> IIGGQDAAHGAWPWMVSLQIFTYHNNRRYHVCGGSLLNSQWLLTAAHCFRIKKKVTDWRLIFGAKEVEWGTNKPVKPPLQERYVEKIIIHEKYSASSEANDIALMKITPPVTCGHFIGPGCLPQFRAGPPRVPQTCWVAGWGFLQENARRTSP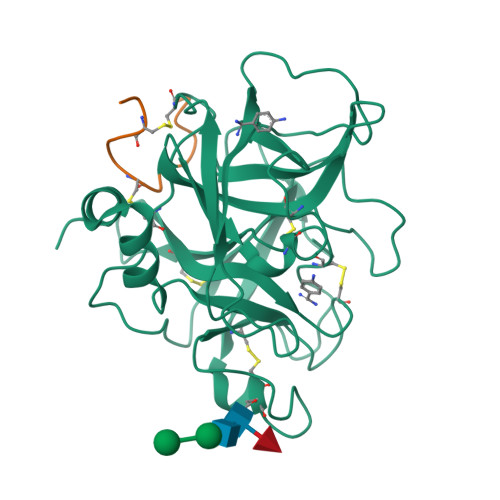MLQEARVDLIDLGLCNSTRWYNGRIRSTNVCAGYPEGKIDTCQGDSGGPLMCKDSAENSYVVVGITSWGVGCARAKRPGVYTSTWSYLNWIASKIGSTAVHMIQLPTASPASTPGAQASSGSVQPSVRPPWFFQQIT;> DNTTCDGPCGVRFRQNRQGGVR> MEKLEVGIYTRAREGEIACGDACLVKRVEGVIFLAVGDGIGHGPEAARAAEIAIASMESSMNTGLVNIFQLCHRELRGTRGAVAALCRVDRRQGLWQAAIVGNIHVKILSAKGIITPLATPGILGYNYPHQLLIAKGSYQEGDLFLIHSDGIQEGAVPLALLANYRLTAEELV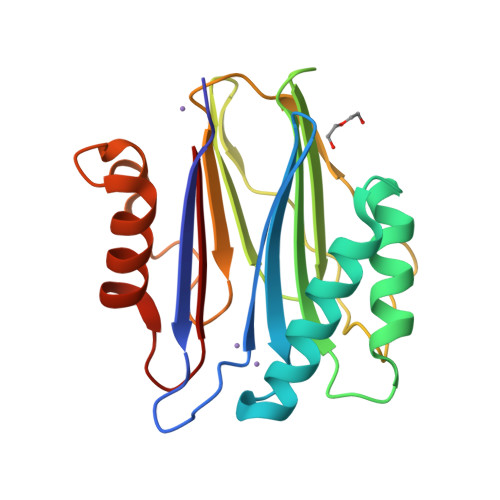RLIGEKYGRRDDDVAVIVAR>[6x]ADTIVAVELDTYPNTDIGDPSYPHIGIDIKS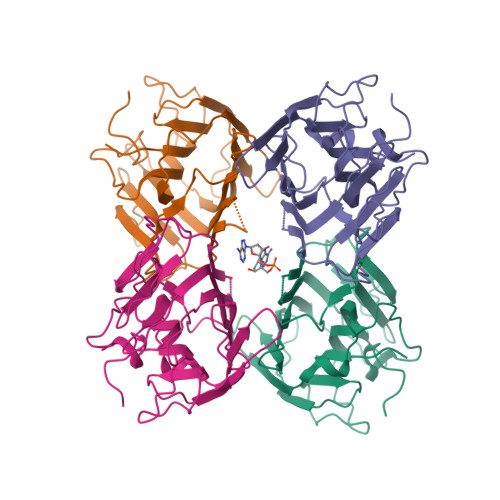VRSKKTAKWNMQNGKVGTAHIIYNSVGKRLSAVVSYPNGDSATVSYDVDLDNVLPEWVRVGLSASTGLYKETNTILSWSFTSKLKSNSTHETNALHFVFNQFSKDQKDLILQGDATTGTDGNLELTRVSSNGSPQGSSVGRALFYAPVHIWESSAVVASFDATFTFLIKSSDSHPADGIAFFISNIDSSIPSGSTGRLLGLFPDAN>[2x]MSQSNRELVVDFLSYKLSQKGYSWSQMAAV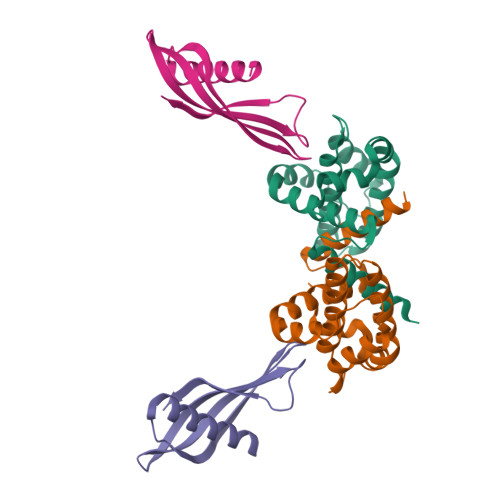KQALREAGDEFELRYRRAFSDLTSQLHITPGTAYQSFEQVVNELFRDGVNWGRIVAFFSFGGALCVESVDKEMQVLVSRIAAWMATYLNDHLEPWIQENGGWDTFVELYGNNAAAESRKGQER;>[2x]SENSLEIEELARFAVDEHNKKENALLEFVRVVKAKEQERNSIFEEFTMYYLTLEAKDGGKKKLYEAKVWVKRDLVFGGPENFKELQEFKPV>[4x]SNAMKDVVIVSAVRTPIGSFGGVFKNTSAVQLGTIAVKEAISRVGLNLSEIDEVIIGNVLQTGLGQNVARQIAINAGIPNSVPSYTVNKLCGSGLKSVQLAAQSITSGENDVVIAGGTENMSQAPYIVPTARFGSKMGNITMVDSMLTDGLIDAFNQYHMGITAENIATKFEFTREMQDKLALESQNKAENAIKNNRFKEEIVPVDVLIRRGKIETIDKDEYPKLGMTFEGLSKLKPAFKKDGTVTAGN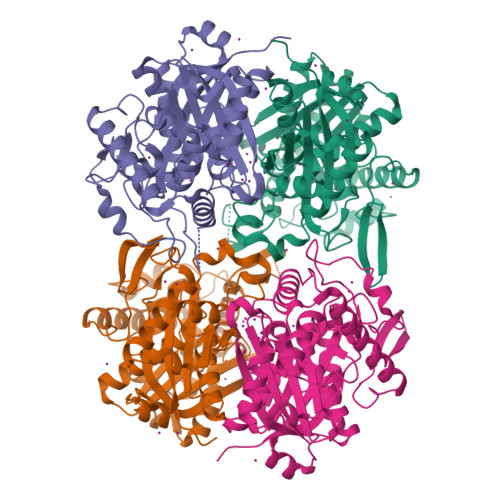ASGINDGAAMLILMSQQKADELGIRPLAKIKSYASAGVEPEVMGTGPIPATRKALKKAGLSINDIDLIEANEAFAAQALAVKNELQIDSSKLNVNGGAIALGHPIGASGARILVTLIYEMQKRKVETGLATLCIGGGQGISMVVSR2-[(3-HYDROXY-2-METHYL-5-PHOSPHONOOXYMETHYL-PYRIDIN-4-YLMETHYL)-AMINO]-2-METHYL-SUCCINIC ACID 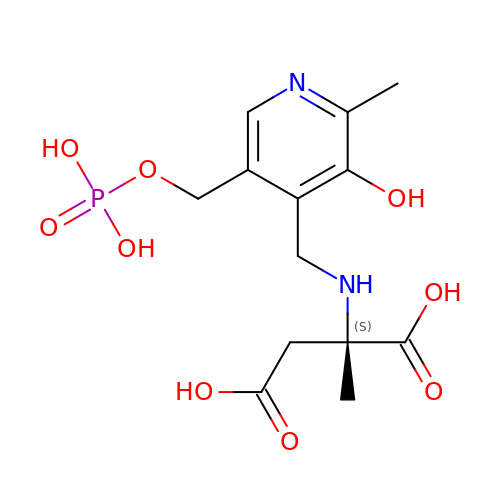| C13 H19 N2 O9 P | ZFKRUCNEKPIDBK-ZDUSSCGKSA-N3-[8-((2S,3S,4R)-2,3,4,5-TETRAHYDROXYPENTYL)-2,4,7-TRIOXO-1,3,8-TRIHYDROPTERIDIN-6-YL]PROPANOIC ACID | C14 H18 N4 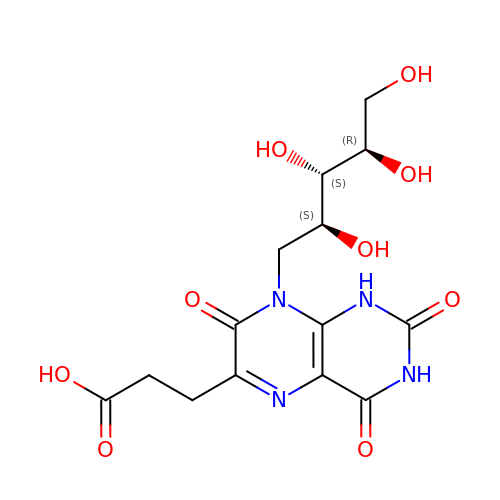O9 | PTYCEIBBGGLADD-PJKMHFRUSA-N>MGSSHHHHHHSSGRENLYFQGMTKPLILASQSPRRKELLDLLQLPYSIIVSEVEEKLNRNFSPEENVQWLAKQKAKAVADLHPHAIVIGADTMVCLDGECLGKPQDQEEAASMLRRLSGRSHSVITAVSIQAENHSETFYDKTEVAFWSLSEEEIWTYIETKEPMDKAGAYGIQGRGALFVKKIDGDYYSVMGLPISKTMRALRHFDIRA[2x]

Maf (for multicopy associated filamentation) proteins represent a large family of conserved proteins implicated in cell division arrest but whose biochemical activity remains unknown. Here, we show that the prokaryotic and eukaryotic Maf proteins exhibit nucleotide pyrophosphatase activity against 5-methyl-UTP, pseudo-UTP, 5-methyl-CTP, and 7-methyl-GTP, which represent the most abundant modified bases in all organisms, as well as against canonical nucleotides dTTP, UTP, and CTP. The protomer structures of the four Maf proteins revealed a large β sheet containing seven β strands (β1 to β7) with two α-helical subdomains on one side and one long α helix on another side. Thus, pyrophosphatase activity of Maf proteins toward canonical and modified nucleotides might provide the molecular mechanism for a dual role of these proteins in cell division arrest and house cleaning.

Previously, BSU28050 has also been reported to exist as a dimer in solution (Minasov et al., 2000). Analysis of the crystal contacts using the quaternary prediction server PISA suggested that the Maf proteins form dimers through multiple interactions between residues located on their C-terminal regions (155–183 in BSU28050, 181–202 in ASMTL-Maf, and 155–193 in YceF). In BSU28050, the pyrophosphate-like molecule is coordinated by the side chains of conserved Ser9 (2.7 Å), Arg14 (2.8 Å and 2.9 Å), and Lys53 (3.0 Å), and its position is similar to that expected for the β-γ-pyrophosphate part of a nucleoside triphosphate substrate. Near the catalytic Asp residue, there are three conserved positive residues (Arg14, Lys53, and Lys82 in BSU28050 and Arg24, Lys65, and Lys100 in ASMTL-Maf) whose side chains have a trigonal orientation in the active site and are arranged similarly to the triphosphate binding site of the E. coli dITPase RdgB (Lys13, Lys53, and Arg87) (Savchenko et al., 2007). In contrast, in the structures of the YhdE-like Maf proteins BSU28050 and ASMTL-Maf, the nucleoside-binding pocket is partially occluded by the guanidine group of an Arg residue (Arg13 in BSU28050, Arg12 in YhdE, Arg29 in YOR111W, and Arg23 in ASMTL-Maf). However, in the structures of BSU28050 and ASMTL-Maf, the side chains of Gln153 and Gln179, respectively, are oriented slightly away from the substrate-binding pocket; therefore, they cannot contribute to base recognition in this conformation. After a minor repositioning of the Arg13 side chain out of base pocket and the Gln153 side chain toward it, the binding pocket of BSU28050 can readily accommodate pyrimidine nucleoside triphosphates in a productive mode. The side chain amide group of Gln153 and the main chain NH group of Ile152 can form three H-bonds to the O2, N3, and O4 groups of thymine, whereas the repositioned guanidine group of Arg13 can make an additional H-bond to the thymine O2.>[12x]MTDFYTIKDAQADLAIAPLNLTVLLAPYSTTPATTLESPTDGSLAIPPGYKSVGHFEKQAGLTLGNEFDSKDIEAYGEPEPIRTIINKRTTTFDFAMYQNQRNVLELIWTQDFSNIQPSEFGGIVLEAPKVPKNIYYRAILVGMDDRNDRPIWLYWLMPKVKLDKLDNQTLNDDNVIEYKPTLKAFRDDVVGYSVAQGFAGPGWRDLVATAGFGEALTALTITPGSPTVTVATGASHTAQLLVEGDNGINYTPDVVFTSSAPDKASVSAAGLVTGVAAGSATITATKGALTATATVTVTA;>MAEFVAAQASVLIVPTLGKGANSFHQKLKEQLQTVRESVDVKIKADTAAMVAEVQATKEMLERDPINIRVETDNNGIKELVKSVTEVRHKYEDLKGDFRRGLTLNLKVVGLSALSQLGPMLASLNTSIVQLSQSSLLLPGIMSGVASSVGAAVVGSRGLTDAFKAQSDASKNVAEAGKQQRDANRAIRDSTRDLNNAIRDAKRNIEDLNAQLRDAPLDEAEAMLNLQEAQYEASQKWGKTAFQQQRDALGLAKAESQLAETRRRNVRLGQDVAEANAKGVNGNDAVVAAQERLTKALEDLAMQTGPIRALNDAMAKLSPNARDFVDQVSSLKGAWDGLRSTVQDRLFDGLGASVQTLAGQDLPILERGLAGIAGAINGNLKTAMSQLATDENKGFLGRIFGNTEEAQNRFSTALKPLLDSFMQLSAVGSDYLPRLSNAFGDVLNRFDGFIERADADGSLDKWINNGLDAMTQLGNSLINVGSIMNTISEAFTGTGGKGLLELLETGTKRLADFLKGAEGQQKLKQFFLDARTELNNWKPLLSQLPGLIKNVATAGQQWANLVLPFLTSAASLLKEHPGLVTAIFTAYMTWRTISPIIGTINLLLSSETGMVGAAKKAGRAVGKGEGLTGKLGVLAGMVGQGGVVMTGLSLVAGFLINEWVTAQNEAAEAVSYHASMISRLKGEMDGLTGSLTTQGLQGKLDAARQWTDIHQTDGKPKDLVAAANSFGVDLPTFMGALTPTNQAARNAVTGKARQTVLDDLNKQGLETVLGKDALNALNLYNQNAAPDKKITNDVLADIATGVNPESKKLFEDAKKSNLIHFNESDLLYGYNKPWGFIPGTDPSGKGLSPVARDAANVSGFVLNDTGNALQVGSDIRSTNEALYGKAVLTPAGQQMFGQFGSPQASFENGSKDAAVRVDTTLQNLPPQFVKDVESNGGHFEELPDGVIIHMRKDRAAQYVTAGSYAGGGFLSGPGTGRSDSMLARVSNGEFITRAASVAKYGRGLFDALNSGTLDPSMLPRFDSGGLVDIFLPGGGTAAPPPTGSANPVDLARGLPRGPAVQSAPANRFDPSPLPTDLLPKPVIPMPDLANPGLYDPATGKYGAAPASAVQQPLKPGVDGDKGETSGPNVPPTDPRSPGYKQPNHGLGGSPGPGNGTPHLTGPGGTPVSPGAASALPSNGGIPGLTPSATDPLGLSGLPKEIQPVTILEQIGEILLSAVLGFFGLDPTYFNIGKRIFTGIKGDKPNEANPGVQSILDGYKNPLADGQNPYVGTSIYDASFDPASQRASNMAELMRGKPYTWGGSSLDGTDCSGLVMYVVDAYEGKEFSGRTGGTGGFASSLPAKGGVIISDPSQAPPGTLRVGWNASHTAGTLPDGRNFESSTFGKPIAVGAGASGYNDPQFTNWAYFPAPGYANGGFLSGAGTGRSDSMLARVSNGEFITRASSVAKYGRSLFDALNAGTVDPGMLPGFADGTPPIPGLPVPQPQTPQQAGPLPDPNGQDAQAAQQVTDTAASALDGVAGAMNGVNMGSSGAIPGADAPDGAQQGKDPRSILGAAPTNTDHNNPALSKGIQGAFSTVGSLASMAASAAMSAGTMGAGAAGASGAAGSGIQAGAQIAGQVATGALNILSSLLVGSAPGSTGTTQSAYGAPVLPQGPPQSSGGGPAVVNNYGDIHTANYDEFYKGQQRREAQQQAPILPVR[3x];>MLSTGPIMETLTLTVGSAFEIPGWKLRGEYPAGTTSHLVFTDAAGGTLGEFEGTVSAKEIHYLQAPDDVKNIPHGANFQLFVTYPSMQPQCLYFGTAIRKEPRYPLSTVVSPEDSAVQYKANFVGQYIGPMWKPMGNGWGSLGIHTHALISEAPSMGPNYSLFSSAAARWLWSMNMDSVTIVVRVLNVGAGKFNVIVCADYQMQTYLGIQFETGISNNKVHVITGDGPLNWGYQGDAVNNTTANGDVYTIKYNDLLDTISCYKGTSLTPLIEASGLDVPHGEGFRYTGLAWNTALLSPGVEPTAWEAKDGV[12x];>MTDFLKIELIGRDGSHWVLSGPGMGQQGVTLNPNLQQFYDAPVKTLYVPGPFGEEYAGKRVQRREIVFSVQAYDEDPDTWSTVDS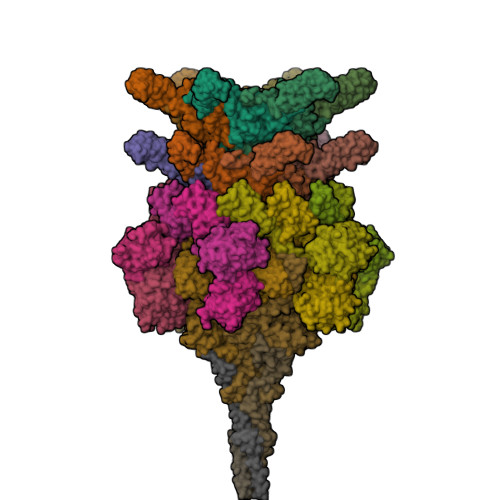LWRWAWDYDEESELRVSTSDGTRFLKVRLMEEPKPYYEKDPHITADNPIVMTVTATFPYWQDEPEELIWTTLSTEDMTRFPVRNDGDVPVWLKWTLTAPGLWILPDFSWGNDMYSRGREDLGRTVAMPELVAGEHVSVDSDPRVQTLIAVNGMPTQNRWKGNDLLYPLMPGKGAEIPVQLKNAPEGGACKLTRPRWYSRPWSRPGVRLNG[6x];>[3x]MANNWTDILAASDGDEWAAFKTIEAQADEVRAGHQALRRAKPLIRLWMNNPDGSEGLVYVGRVDYDDTIRGSFPFKNNTPSQGVLELRDDNYLAVWLKQLPNNPELKKNVVITVDFYGGKKRWSGLLDKWTIKSKEHVKYLEVTFNDDLTMLQYLLCPPNPALPIPVLQFPRIFGIAGPAKWAISTLIFINLFRVQGNLWTLPDDPFNLESWDDILDWSDWQCFVKSNSFLLDDSSVWTFLSSRMNPVDSIIADALDDAQLTITYRRVLTDDGETAEGFPGAHGIKNGALVFEIVDNSNATALEGTFFSGTIVDGFARSVLLYGGGFVEDTLSVVSDDQTLQPDEYYQSGWLATMAKMPWLVVRDNEWTPIESSDLSWGPAKNVSVIVGGDNPAADAIAKLIIETTGNLLGYFLLGGFSSAGTIAADIIMPFLVGTIAAWLQWKNTGRATELGWVHYWELYQQGAETNSWSLAALAALRGGFLVGRSETVHLMALHDSWIIPGLHIDIGQRMGSTVNSKGVENIVWVNQLEEMTAAWDNSAGQTMPLSWVLKAGKSDRAMSIGERVARLAKKMSEALNNVGVHIVQS;>MTMPNGSGGLDPGAWLSHWVNQADLSSLAGRTEDEVRAYFENLVQADSGWGDASNTFFNLILGGFQNLSEFVTLIVQAVTGAPGGLTDLQAFLTERWGDLADAFQAVANLIDAIAGEVGSSLADAIAKLATFLTELSPLNAGMLFGLIGTNHLPLLSVSHIANINPELLVNAGFDSDVSVVDNPYWDWDGTVGRTAPLGAVKVVADGTIKDLLSGPDAIPVVEGQKLNVSAWLKYSGLVAGAGAGSIRLSGTAYSADGEVVAYPDFGGIPDGASGTSDWTQVTGQYVVPAGVTQFRLRLSVRENATGGTVWFDDCSVKKAGLLPQGLVDGLVQALSDLLTWLESLVDNVLSALGLDPIGTIVDKILDLADEFGDWLGATEDTAANLSNLLTKLLSDPASVIGPLAQSMITGLTGALGNLNTAINQIGDVLVGTVVTPINSAISNVIDWFNSLLNFQDTTTSNQINQQNFQIATLASGIKKQQWECRYSTAFVTFPEMFCDWGFALGGTTGAQSTGTAHTHTLNTDGLAALQIQILPAGYAIGGYIGISDTTIVDTIAMKMYKETSSAINNVYLEVFREDSTGALTSVGSVDVSGQLTTASDYVEATLPAGVIVNAGERYVVRMRNATTVGNRVGVSVMKELVGGRELSIRTETATDSNKTFYTPSEVLTAQGVSVIMPWAMMAAKNLATTDQSFSDDFNRSAMGGLWFLKSDTGTNQVGVSGGRAAFSGLTDGNQNALYIRPTAGDKQWVEATLYETGIAASGAREGLLMHANRDLSQVVYLGVNLNTAKIYTGPWNSLTERASVSTTGNDVLWQMYFDPATAAYTVLKNGQASGLTWTDSGSVVAHGPNYRFGGLRISRATFFNAGRIDNWTLKDWA[3x]>[3x]MKEDQVVAEEPGFQDEEESLFQDIDLLQKHGINVADIKKLKSVGICTIKGIQMTTRRALCNVKGLSEAKVDKIKEAANKLIEPGFLTAFEYSEKRKMVFHITTGSQEFDKLLGGGIESMAITEAFGEFRTGKTQLSHTLCVTAQLPGAGGYPGGKIIFIDTENTFRPDRLRDIADRFN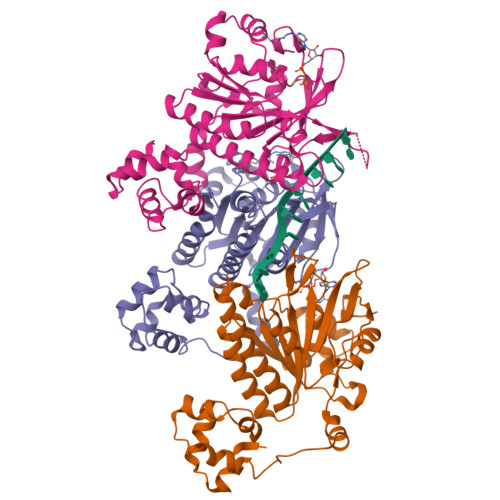VDHDAVLDNVLYARAYTSEHQMELLDYVAAKFHEEAGIFKLLIIDSIMALFRVDFSGRGELAERQQKLAQMLSRLQKISEEYNVAVFVTNQMTADPGATMTFQADPKKPIGGHILAHASTTRISLRKGRGELRIAKIYDSPEMPENEATFAITAGGIGDAKE> MTDQPDLFGLAPDAPRPIIPANLPEDWQEALLPEFSAPYFHELTDFLRQERKEYTIYPPAPDVFNALRYTPLGEVKVLILGQDPYHGPNQAHGLSFSVRPGVRVPPSLRNIYKELTEDIPGFVAPKHGYLRSWAEQGVLLLNAVLTVRAGQANSHQGKGWEHFTDAVIKAVNAK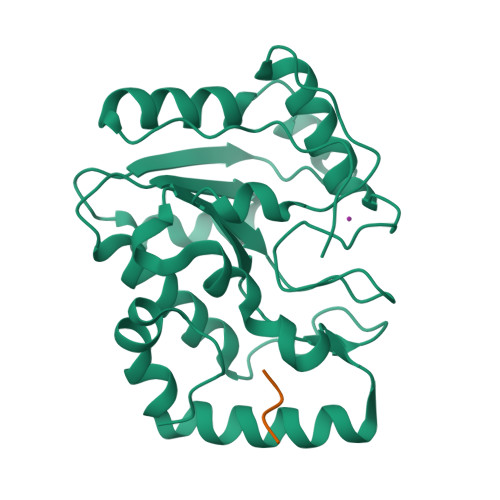EERVVFILWGSYARKKKKLITGKNHVVIESGHPSPLSEQYFFGTRPFSKTNEALEKAGRGPVEWQLPATVTEELEHHHHHH;> DDFPPEEDDLPF>[6x]N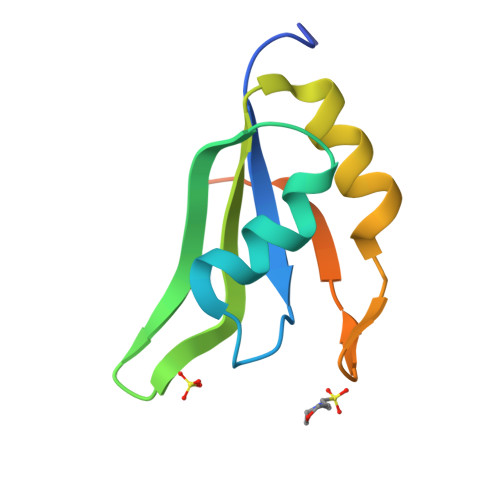TENKSQPKRLHVSNIPFRFRDPDLRQMFGQFGKILDVEIIFNERGSKGFGFVTFENSADADRAREKLHGTVVEGRKIEVNNATARVMTNKKTVNPYTNG> AFVVTDNCIKCKYTNCVEVCPVDCFYEGPNFLVIHPDECIDCALCEPEC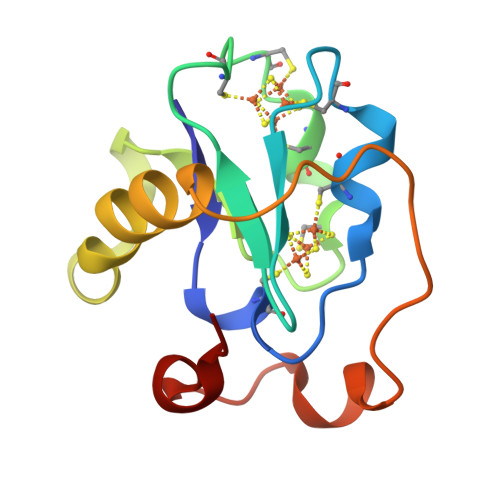PAQAIFSEDEVPEDMQEFIQLNAELAEVWPNITEKKDPLPDAEDWDGVKGKLQHLER> MVQKESQATLEERESELSSNPAASAGASLEPPAAPAPGEDNPAGAGGAAVAGAAGGARRFLCGVVEGFYGRPWVMEQRKELFRRLQKWELNTYLYAPKDDYKHRMFWREMYSVEEAEQLM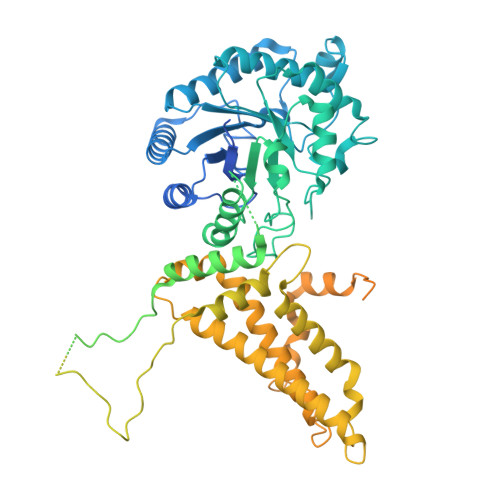TLISAAREYEIEFIYAISPGLDITFSNPKEVSTLKRKLDQVSQFGCRSFALLFDDIDHNMCAADKEVFSSFAHAQVSITNEIYQYLGEPETFLFCPTEYCGTFCYPNVSQSPYLRTVGEKLLPGIEVLWTGPKVVSKEIPVESIEEVSKIIKRAPVIWDNIHANDYDQKRLFLGPYKGRSTELIPRLKGVLTNPNCEFEANYVAIHTLATWYKSNMNGVRKDVVMTDSEDSTVSIQIKLENEGSDEDIETDVLYSPQMALKLALTEWLQEFGVPHQYSSRQVAHSGAKASVVDGTPLVAAPSLNATTVVTTVYQEPIMSQGAALSGEPTTLTKEEEKKQPDEEPMDMVVEKQEETDHKNDNQILSEIVEAKMAEELKPMDTDKESIAESKSPEMSMQEDCISDIAPMQTDEQTNKEQFVPGPNEKPLYTAEPVTLEDLQLLADLFYLPYEHGPKGAQMLREFQWLRANSSVVSVNCKGKDSEKIEEWRSRAAKFEEMCGLVMGMFTRLSNCANRTILYDMYSYVWDIKSIMSMVKSFVQWLGCRSHSSAQFLIGDQEPWAFRGGLAGEFQRLLPIDGANDLFFQPPPLTPTSKVYTIRPYFPKDEASVYKICREMYDDGVGLPFQSQPDLIGDKLVGGLLSLSLDYCFVLEDEDGICGYALGTVDVTPFIKKCKISWIPFMQEKYTKPNGDKELSEAEKIMLSFHEEQEVLPETFLANFPSLIKMDIHKKVTDPSVAKSMMACLLSSLKANGSRGAFCEVRPDDKRILEFYSKLGCFEIAKMEGFPKDVVILGRSL>[6x]TLLHPLL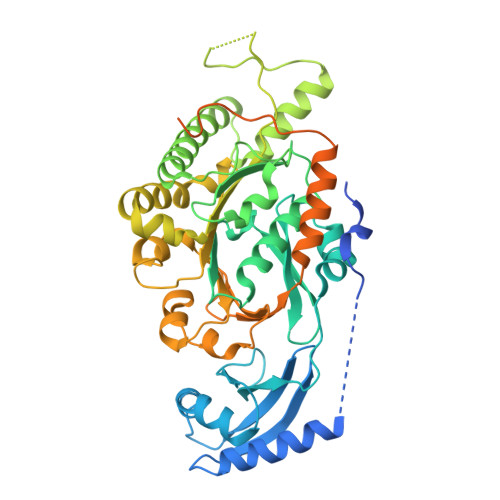MRNGDSRPLHKPTTPLPSLDLLTPPPSEVEPVDTFALEQMARLVEARLADFRIKADVVNYSPGPVITRFELNLAPGVKAARISNLSRDLARSLSTVAVRVVEVIPGKPYVGLELPNKKRQTVYLREVLDNAKFRDNPSPLTVVLGKDIAGEPVVADLAKMPHLLVAGTTGSGASVGVNAMILSMLYKAQPEDVRFIMIDPKMLELSVYEGIPHLLTEVVTDMKDAANALRWCVNEMERRYKLMSALGVRNLAGYNEKIAEADRMMRPIPDPYWKPGDSMDAQHPVLKKEPYIVVLVDEFADLMMTVGKKVEELIARLAQKARAAGIHLVLATQRPSVDVITGLIKANIPTRIAFTVSSKIDSRTILDQAGAESLLGMGDMLYSGPNSTLPVRVHGAFVRDQEVHAVVQDWKARGRPQYVDGITSDSESEGGAGGFDGAEELDPLFDQAVQFVTEKRKASISGVQRQFRIGYNRAARIIEQMEAQGIVSEQGHNGNREVLAPPPFD>[8x]MTKPTSAGQADDALVRLA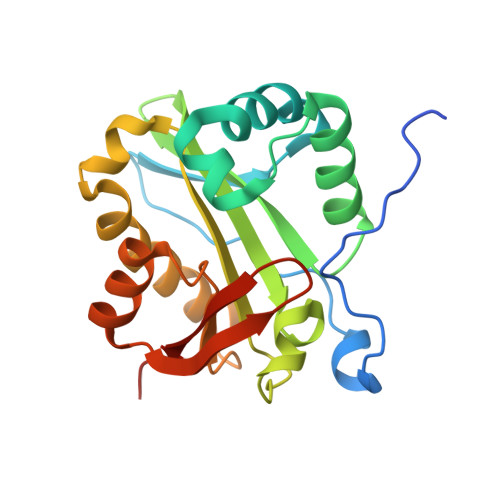RERFDLPDQVRRLARPPVPSLEPPYGLRVAQLTDAEMLAEWMNRPHLAAAWEYDWPASRWRQHLNAQLEGTYSLPLIGSWHGTDGGYLELYWAAKDLISHYYDADPYDLGLHAAIADLSKVNRGFGPLLLPRIVASVFANEPRCRRIMFDPDHRNTATRRLCEWAGCKFLGEHDTTNRRMALYALEAPTTAA>[4x]MDAVAVYHGKISRETGEKLLLATGLDGSYLLRDSESVPGVYC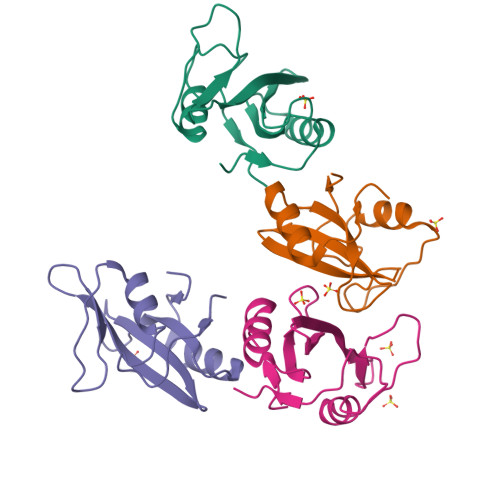LCVLYHGYIYTYRVSQTETGSWSAETAPGVHKRYFRKIKNLISAFQKPDQGIVIPLQYPVEK>AMLSPEALTTAVDAAQQAIALADTLDVLARVKTEHLGDRSPLALARQALAVLPKEQRAEAGKRVNAARNAAQRSYDERLATLRAERDAAVLVAEGIDVTLPSTRVPAGARHPIIMLAEHVADTFIAMGWELAEGPEVETEQFNFDALNFPADHPARGEQDTFYIAPEDSRQLLRTHTSPVQIRTLLARELPVYIISIGRTFRTDELDATHTPIFHQVEGLAVDRGLSMAHLRGTLDAFARAEFGPSARTRIRPHFFPFTEPSAEVDVWFANKIGGAAWVEWGGCGMVHPNVLRATGIDPDLYSGFAFGMGLERTLQFRNGIPDMRDMVEGDVRFSLPFGVGA[2x];>QSNAMRLPYSWLREVVAVGASGWDVTPGELEQTLLRIGHEVEEVIPLGPVDGPVTVGRVADIEELTGYKKPIRACAVDIGDRQYREIICGATNFAVGDLVVVALPGATLPGGFTISARKAYGRNSDGMICSAAELNLGADHSGILVLPPGAAEPGADGAGVLGLDDVVFHLAITPDRGYCMSVRGLARELACAYDLDFVDPASNSRVPPLPIEGPAWPLTVQPETGVRRFALRPVIGIDPAAVSPWWLQRRLLLCGIRATCPAVDVTNYVMLELGHPMHAHDRNRISGTLGVRFARSGETAVTLDGIERKLDTADVLIVDDAATAAIGGVMGAASTEVRADSTDVLLEAAIWDPAAVSRTQRRLHLPSEAARRYERTVDPAISVAALDRCARLLADIAGGEVSPTLTDWRGDPPCDDWSPPPIRMGVDVPDRIAGVAYPQGTTARRLAQIGAVVTHDGDTLTVTPPSWRPDLRQPADLVEEVLRLEGLEVIPSVLPPAPAGRGLTAGQQRRRTIGRSLALSGYVEILPTPFLPAGVFDLWGLEADDSRRMTTRVLNPLEADRPQLATTLLPALLEALVRNVSRGLVDVALFAIAQVVQPTEQTRGVGLIPVDRRPTDDEIAMLDASLPRQPQHVAAVLAGLREPRGPWGPGRPVEAADAFEAVRIIARASRVDVTLRPAQYLPWHPGRCAQVFVGESSVGHAGQLHPAVIERSGLPKGTCAVELNLDAIPCSAPLPAPRVSPYPAVFQDVSLVVAADIPAQAVADAVRAGAGDLLEDIALFDVFTGPQIGEHRKSLTFALRFRAPDRTLTEDDASAARDAAVQSAAERVGAVLRG[2x]

AaRSs catalyze the attachment of the correct amino acid to its cognate tRNA which then is used in protein synthesis on ribosomes. Phylogenetically phenylalanyl-tRNA synthetase (PheRS), belongs to the class II aaRSs, and it is a dimer of heterodimers (αβ)2, containing two α- (PheS) and two β- (PheT) subunits. Structural studies of PheRS have shown that the α subunit binds L-Phe and ATP and is responsible for esterification catalysis. At the same time, the β subunit is involved in the recognition of the cognate tRNA molecule and editing of mis-charged tRNA.

The protein-fragment interactions were analyzed using crystal structures for five of those fragments complexed with MtPheRS/tRNAPhe (DDD00107555 (D-555), DDD01008876 (D-876), DDD00805735 (D-735), DDD00079004 (D-004) and DDD00067116 (D-116)). All five fragments occupy the L-Phe site in the α subunit of the heterotetramer. The fragments’ orientation in these structures is very similar to the L-Phe substrate, however there are subtle differences in orientation and details of interactions. PIEDA showed that the phenyl ring or the bicyclic core of the fragments interact with residues αPhe255 and αPhe257 through hydrophobic interaction. A strong Π-cation interaction between the imidazolidinedione core of D-876 and αArg201 is observed. The carbonyl oxygen of the imidazolidinedione core interacts with αGln215 of MtPheRS through hydrogen bond. The top-ranking fragment D-876 maintains all the critical interactions and makes additional interactions with residues αArg201, αGln215, αGly309 and αArg312. In accordance with this, binding of D-876 fragment exhibited highest interaction energy (−93.6 kcal/mol) and ligand efficiency score (5.2). However, the auxiliary pocket in the structures of PheRS with bound fragments was completely unoccupied offering an opportunity for fragment growth by adding hydrophobic substituents to explore the auxiliary pocket of MtPheRS.> MRCIGISNRDFVEGVSGGSWVDIVLEHGSCVTTMAKNKPTLDFELIETEAKQPATLRKYCIEAKLTNTTTDSRCPTQGEPSLNEEQDKRFVCKHSMVDRGWGNGCGLFGKGGIVTCAMFTCKKNMKGKVVQPENLEYTIVITPHSGEEHAVGNDTGKHGKEIKITPQSSITEAELTGYGTVTMECSPRTGLDFNEMVLLQMENKAWLVHRQWFLDLPLPWLPGADTQGSNWIQKETLVTFKNPHAKKQDVVVLGSQEGAMHTALTGATEIQMSSGNLLFTGHLKCRLRMDKLQLKGMSYSMCTGKFKVVKEIAETQHGTIVIRVQYEGDGSPCKIPFEIMDLEKRHVLGRLITV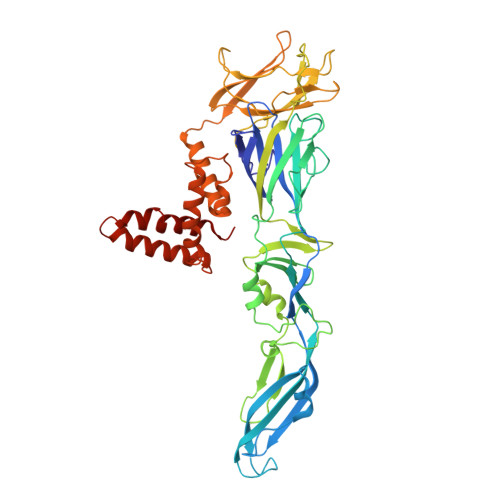NPIVTEKDSPVNIEAEPPFGDSYIIIGVEPGQLKLNWFKKGSSIGQMIETTMRGAKRMAILGDTAWDFGSLGGVFTSIGKALHQVFGAIYGAAFSGVSWIMKILIGVIITWIGMNSRSTSLSVSLVLVGVVTLYLGVMVQA7-(3-{[4-(4-acetylpiperazin-1-yl)phenoxy]methyl}-1,5-dimethyl-1H-pyrazol-4-yl)-3-{3-[(naphthalen-1-yl)oxy]propyl}-1-[(pyridin-3-yl)methyl]-1H-indole-2-carboxylic 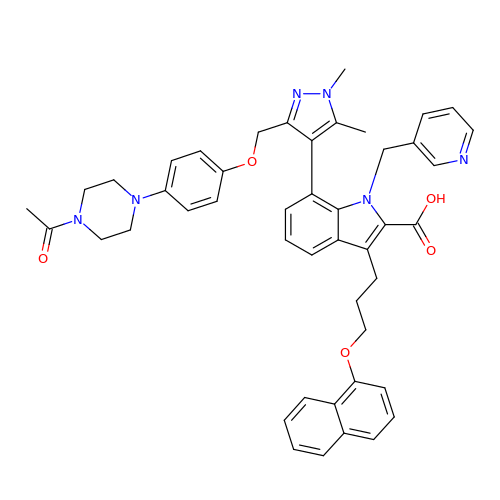acid | C46 H46 N6 O5 | VKKQBUSCPZGZBT-UHFFFAOYSA-N> MASILDCPIVSVNARVWRFWSFVLKHDAMRYISIIPVTVMTFFMFTDLCRSWGNIQELIIKAYFAVLYFNAVLRTLILVKDRKLYENFMQGISNVYFEISHIDDHKIQSLLKSYTVRARMLSISNLALGAIISTCFVVYPIFTGERGLPYGMFIPGLDSFRSPHYEIIYIVQVVLTFPGCCMYIPFTSFFASTTLFGLVQIKTLQRQLQTFKDNINSQ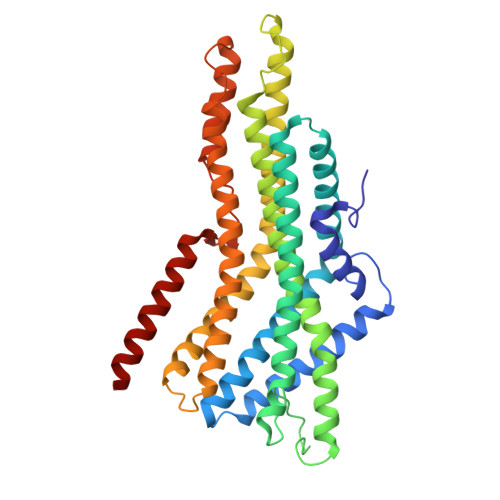DKEKVKAKVVKLIEDHKRIITYVSELNSLVTYICFVEFLSFGMMLCALLFLLNVIENHAQIVIVAAYIFMIISQIFAFYWHANEVREESMNLAEAAYSGPWVELDNSIKKKLLLIILRAQQPLEITVGNVYPMTLEMFQSLLNASYSYFTLLRRVYN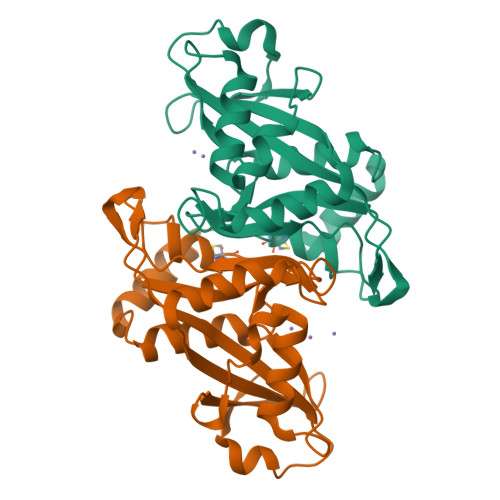>[2x]MAESRSPDRGAKEDKPRPRNISREESLQLEGYKHACHALLHAPSQAKLFDRVPIRRVLLMMMRFDGRLGFPGGFVDTRDISLEEGLKRELEEELGPALATVEVTEDDYRSSQVREHPQKCVTHFYIKELKLEEIERIEAEAVNAKDHGLEVMGLIRVPLYTLRDRVGGLPAFLCNNFIGNSKSQLLYALRSLKLLREDQIQEVLKASHRLQY> MLEKVETFDMNRVIDEFDEMTRNAHQVQKQTLKEILLKNQSAIYLQNCGLNGNATDPEEAFKSMVPLVTDVELEPYIKRMVDGDTSPILTGHPVPAISLSSGTSQGRPKFIPFTDELMENTLQLFRTAFAFRNRDFPIDDNGKALQFIFSSKQYISTGGVPVGTATTNVYRNPNFKAGMKSITSPSCSPDEVIFSPDVHQALYCHLLSGILFRDQVQYVFAVFAHGLVHAFRTFEQVWEEIVTDIKDGVLSNRITVPSVRTAMSKLLTPNPELAETIRTKCMSLSNWYGLIPALFPNAKYVYGIMTGSMEPYVPKLRHYAGDLPLVSHDYGSSEGWIAANVTPRL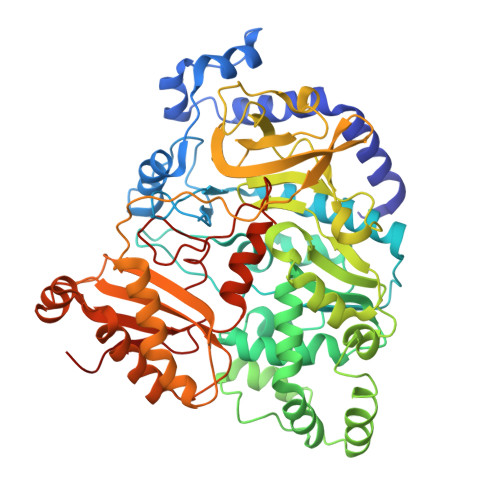SPEEATFAVIPNLGYFEFLPVSETGEGEEKPVGLTQVKIGEEYEVVITNYAGLYRYRLGDVVKVIGFYNNTPQLKFICRRNLILSINIDKNTERDLQLSVESAAKRLSEEKIEVIDFSSYIDVSTDPGHYAIFWEISGETNEDVLQDCCNCLDRAFIDAGYVSSRKCKTIGALELRVVAKGTFRKIQEHFLGLGSSAGQFKMPRCVKPSNAKVLQILCENVVSSYFSTAF>[2x]LTCVKSNSIWFPTSEDCPDGQNLCFKRWQYISPRMYDF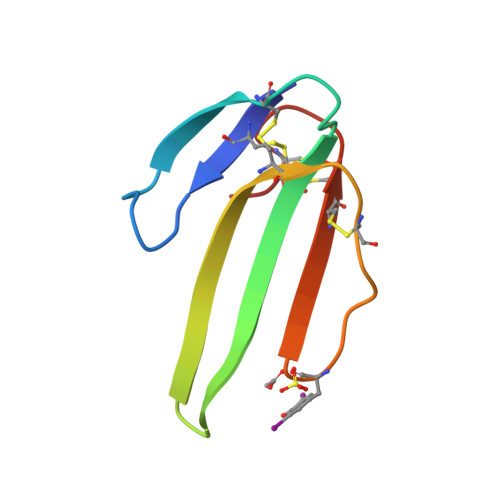TRGCAATCPKAEYRDVINCCGTDKCNK> GLIVDTRDVEERVHVMRKTELAPTVAHGVFNPEFGPAALSNKDPRLNEGVVLDEVIFSKHKGDTKMSAEDKALFRRCAADYASRLHSVLGTANAPLSIYEAIKGVDGLDAMEPDTAPGLPWALQGKRRGALIDFENGTVGPEVEAALKLMEKREYKFACQTFLKDEIRPMEKVRAGKTRIVDVLPVEHILYTRMMIGRFCAQMHSNNGPQIGSAVGCNPDVDWQRFGTHFAQYRNVWDVDYSAFDANHCSDAMNIMFEEVFRTEFGFHPNAEWILKTLVNTEHAYENKRITVEGGMPSGCSATSIINTILNNIYVLYALRRHYEGVELDTYTMISYGDDIVVASDYDLDFEALKPHFKSLGQTITPADKSDKGFVLGHSITDVTFLKRHFHMDYGTGFYKPVMASKTLEAILSFARRGTIQEKLISVAGLAVHSGPDEYRRLFEPFQGLFEIPSYRSLYLRWVNAVCGD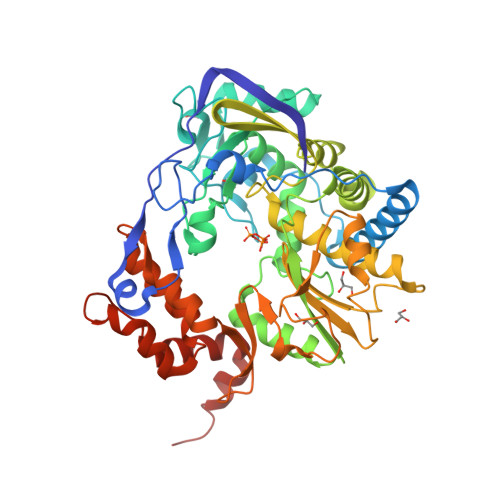AAAALEHHHHHH> MRAEGLGGLERFCSPGKG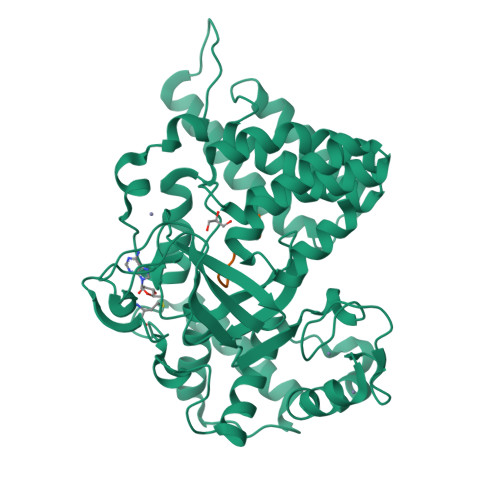RGLRALQPFQVGDLLFSCPAYAYVLTVNERGNHCEYCFTRKEGLSKCGRCKQAFYCNVECQKEDWPMHKLECSPMVVFGENWNPSETVRLTARILAKQKIHPERTPSEKLLAVKEFESHLDKLDNEKKDLIQSDIAALHHFYSKHLGFPDNDSLVVLFAQVNCNGFTIEDEELSHLGSAIFPDVALMNHSCCPNVIVTYKGTLAEVRAVQEIKPGEEVFTSYIDLLYPTEDRNDRLRDSYFFTCECQECTTKDKDKAKVEIRKLSDPPKAEAIRDMVRYARNVIEEFRRAKHYKSPSELLEICELSQEKMSSVFEDSNVYMLHMMYQAMGVCLYMQDWEGALQYGQKIIKPYSKHYPLYSLNVASMWLKLGRLYMGLEHKAAGEKALKKAIAIMEVAHGKDHPYISEIKQEIESH;> HSSHLKSKKGQ>GH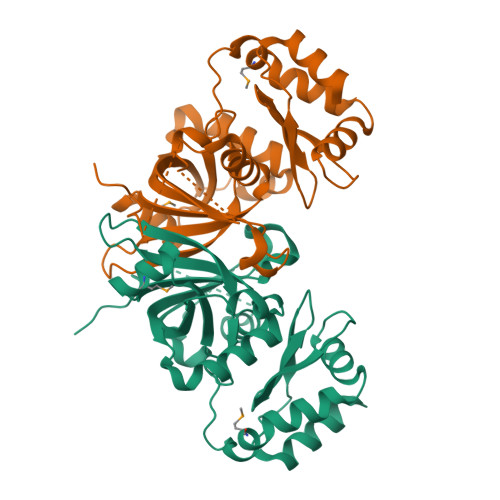MLDVAPPVITPRGTKIEPSAGAPFEAVRVARDVLHTSRTAALATLDPVSGYPYTTATNIGIEPDGTPFFFAAGLTLHARNMETDARISVTLAPFGKGDALTLPRLTLVGRADRIGPDEVPLAIARYIARYPKAKLYLSLPDTRLYRLRTEGVQINGGPARNASNITPADLRTDLSGAEELMAAAESEATRLNAIKGEASRLAVLAGAKTGRWKITSIDPDGIDLASASDLARLWFAERVETLKQFEKALAQLLKGS[2x]> FQTQKPLKSTSLSLFYKKVYRLAYLRLNTLCERLLSEHPELEHIIWTLFQHTLQNEYELMRDRHLDQIMMCSMYGICKVKNIDLK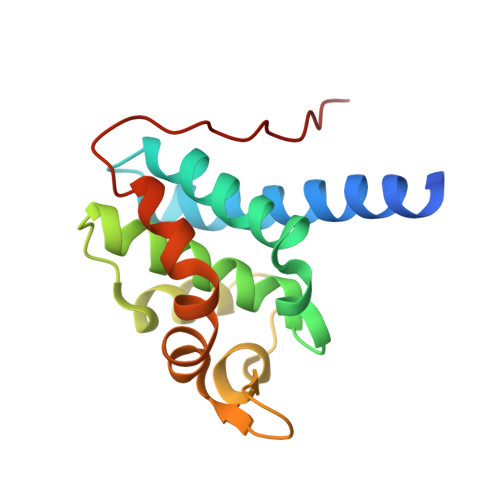FKIIVTAYKDLPHAVQETFKRVLIKEEEYDSIIVFYNSVFMQRLKTNILQYASTRPPTLSPIPHIPR> MEYVKNVVCPFCGTLCDDIICKVEGNEIVGTINACRIGHSKFVHAEGAMRYKKPLI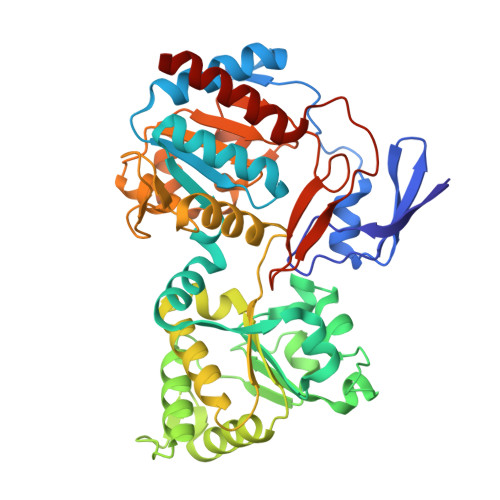RKNGEFVEVSYDEAIDKAAKILAESKRPLMYGWSCTECEAQAVGVELAEEAGAVIDNTASVCHGPSVLALQDVGYPICTFGEVKNRADVVVYWGCNPMHAHPRHMSRNVFARGFFRERGRSDRTLIVVDPRKTDSAKLADIHLQLDFDRDYELLDAMRACLLGHEILYDEVAGVPREQIEEAVEVLKNAQFGILFFGMGITHSRGKHRNIDTAIMMVQDLNDYAKWTLIPMRGHYNVTGFNQVCTWESGYPYCVDFSGGEPRYNPGETGANDLLQNREADAMMVIASDPGAHFPQRALERMAEIPVIAIEPHRTPTTEMADIIIPPAIVGMEAEGTAYRMEGVPIRMKKVVDSDLLSDREILERLLEKVREYKASK> MWNPIVNVDITLNTAGTTREGFGLPLFLASTDNFEERVRGYTSLTEVAEDFDENTAAYKAAKQLWSQTPKVTQLYIGRRAMQYTVSIPNAVTESTDYSITVAAGGGISQPYQYTAQAEDTAENVLQQFKTQIEADPTIKDKVSV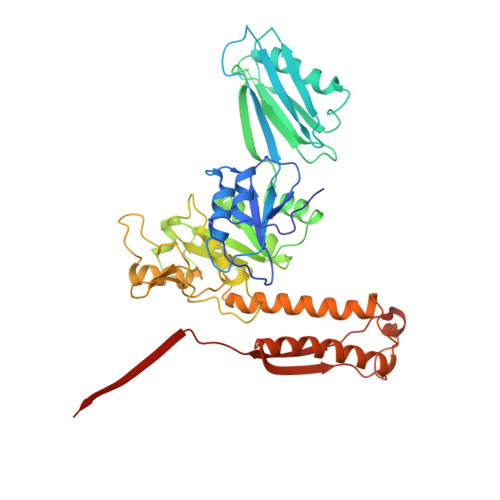NVTGSNGSATMIITKAGDNDFVKVTTTAQTVYIASTTADTASTALAAIEAYSTDWYFIAAEDRTQQFVLAMASEIQARKKIFFTANSDVTALQGTELASANDVPAQLAKNMYTRTVCLWHHAAAEDYPEMAYIAYGAPYDAGSIAWGNAQLTGVAASLQPSNQRPLTSIQKSALDVRHCNFIDLDGGVPVVRRGITSGGEWIDIVRGVDWLESDLKTSLRDLLINQKGGKITYDDTGITRIRQVIETSLQRAVNRNFLSSYTVNVPKASQVALADKKARILKDVTFAGILAGAILDVDLKGTVAYE>[4x]AEEFPVPNGFESAYREVDGVKLHYVKGGQGPLVMLVHGFGQTWYEWHQLMPELAKRFTVIAPDLPGLGQSEPPKTGYSGEQVAVYLHKLARQFSPDRPFDLVAHDIGIWNTYPMVVKNQADIARLVYMEAPIPDARIYRFPAFTAQGESLVWHFSFFAADDRLAETLIAGKERFFLEHFIKSHASNTEVFSERLLDLYARSYAKP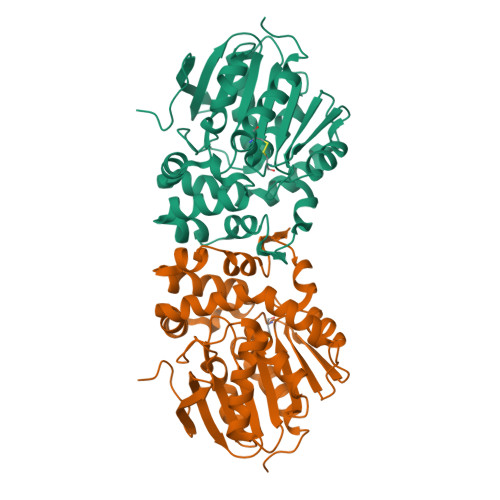HSLNASFEYYRALNESVRQNAELAKTRLQMPTMTLAGGGAGGMGTFQLEQMKAYAEDVEGHVLPGCGHWLPEECAAPMNRLVIDFLSRGRHHHHHH> MRCNERNKKKAIFSNDDFSGEDTLMEDHLQLREKLSEDIEMIKASLKNNLVCSTLNDNEILTLSNYMQFFVFKGGDLVIKQGEKGSYFFIINSGKFDVYVNDKKVKSMGKGSSFGEAALIHNTQRSATIMAETDGTLWGVQRSTFRATLKQLSNRNFNENRSFIDSVSVFDMLTEAQKNMITNACVIQMFKPGETIVKQGDYGDVLFILKEGKATVFINDKEIRVLNKGSYFGERALLYDEPRSATIIAKEPTACASICRKLLNIVLGNLQVVLFRNIMTEALQQSEIFRQFSAEQLNDLADTAIVRDYPANYHILHKDKVKSVKYLIVLEGKVELFLDDESIGILTRGKSFGDQYVLNQKQKFRHTVKSLDVCKIALITESCLADCLGDNNIDASIDHNNKKSIIKKMYIFRYLSEQQC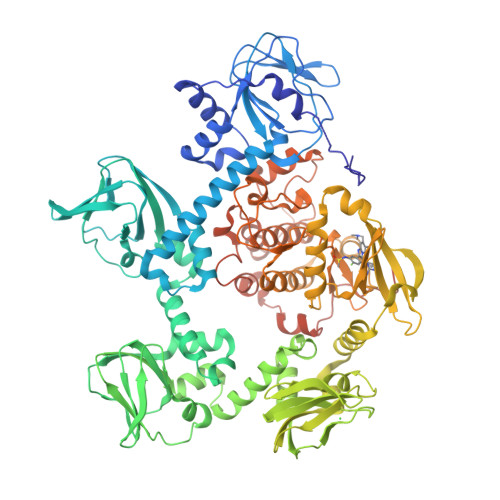NLLIEAFRTTRYEEGDYIIQEGEVGSRFYIIKNGEVEVTKNGKRLRTLGKNDYFGERALLYDEPRTASIISKATSVECWFVDKSVFLQIIQGPMLTHLEERIKMQDTKVEMHELETERIIGRGTFGTVKLVHHKPTQIRYALKCVSKRSIISLNQQNNIKLEREITAENDHPFIIRLVRTFKDSNCFYFLTELVTGGELYDAIRKLGLLSKPQAQFYLGSIILAIEYLHERNIVYRDLKPENILLDKQGYVKLIDFGCAKKIQGRAYTLVGTPHYMAPEVILGKGYGCTVDIWALGVCLYEFICGPLPFGNDQEDQLEIFRDILTGQLTFPDYVSDQDSINLMKRLLCRLPQGRIGCSINGFKDIKEHAFFGNFNWDKLAGRLLEPPLVSKGETYAEDIDIKQIEEEDALNEGEPLDGDDSWDVDF> MHHHHHHSSGRENLYFQGMSFEITE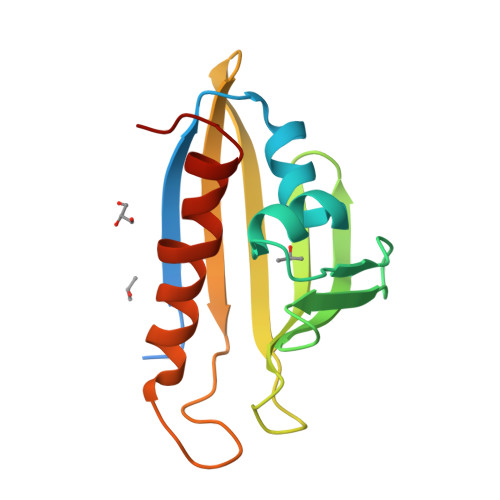EYYVPPEVLFNAFTDAYTLTRLSRGSLAEVDLKVGGKFSLFSGSILGEFTEITKPHKIVEKWKFRDWNECDYSTVTVEFISVKENHTKLKLTHNNIPASNKYNEGGVLERCKNGWTQNFLHNIEVILGYPKKK> GPDLPEGYEQRTTQQGQVYFLHTQTGVSTWHDPRVPRDLSNINCEELGPLPPGWEIRNTATGRVYFVDHNNRTTQFTDPRLSANLHLVLNRQNQLKDQQQQQVVSLCPDDTECLTVPRYKRDLVQKLKILRQELSQQQPQAGHCRIEVSREEIFEESYRQVMKMRPKDLWKRLMIKFRGEEGLDYGGVAREWLYLLSHEMLNPYYGLFQYSRDDIYTLQINPDSAVNPEHLSYFHFVGRIMGMAVFHGHYIDGGFTLPFYKQLLGKSITLDDMELVDPDLHNSLVWILENDITGVLDHTFCVEHNAYGEIIQHELKPNGKSIPVNEENKKEYVRLYVNWRFLRGIEAQFLALQKGFNEVIPQHLLKTFDEKELELIICGLGKIDVNDWKVNTRLKHCTPDSNIVKWFWKAVEFFDEERRARLLQFVTGSSRVPLQGFKALQGAAGPRLFTIHQIDACTNNLPKAHTCFNRIDIPPYESYEKLYEKLLTAIEETCGFAVE

The structure of SMURF1 is typical of a NEDD4 subfamily member, with a N-terminal C2 domain for cellular membrane localization, WW domains for target recognition, and a catalytic HECT domain that binds E2 and mediates target ubiquitylation through a surface-protruding catalytic cysteine. At the cellular level, SMURF1 acts as a negative regulator of bone morphogenetic protein (BMP) signaling, which modulates cell migration, proliferation, and apoptosis. Ubiquitin transfer requires a motion facilitated by a flexible hinge that connects the HECT domain N- and C-lobes. To gain structural insights into the mechanism of selective inhibition, we crystallized the HECT domains of both SMURF1 and SMURF2, without and with a representative SMURF1 inhibitor, compound-8 (Cpd-8), and determined structures at 2.05–2.75 Å resolution.

Although SMURF1 and SMURF2 share a high degree of protein sequence homology (86% identity), we identified potent inhibitors that were selective for SMURF1 over SMURF2, which were structurally distinct from those reported in prior studies. The structure of SMURF2 in complex with Cpd-8 demonstrated binding of the same cryptic cavity as the SMURF1-inhibitor complex. However, in contrast to SMURF1, inhibitor binding did not elongate the SMURF2 αH10, and the invariant glycine (G628) stems the hinge in both the inhibitor-bound and -unbound forms. SMURF1 R686 is conserved in SMURF2 as R680, but SMURF1 D636 is replaced with G630 in SMURF2, meaning that the network of non-covalent bonds stabilizing the elongated αH10 in SMURF1 cannot be formed in SMURF2. Consistent with this, SMURF2 was not inhibited by Cpd-8. The resistance of SMURF2 to inhibition is likely conferred by G630, which, in the presence of compound, does not form the bond network required to lock the elongated αH10. To examine whether introducing the residues required for the formation of the stabilizing bond network would render SMURF2 sensitive to inhibition, we engineered SMURF2 with a G630D substitution (named SMURF1lation). However, the G630D SMURF2 was susceptible to inhibition by Cpd-8.MIMOSINE | C8 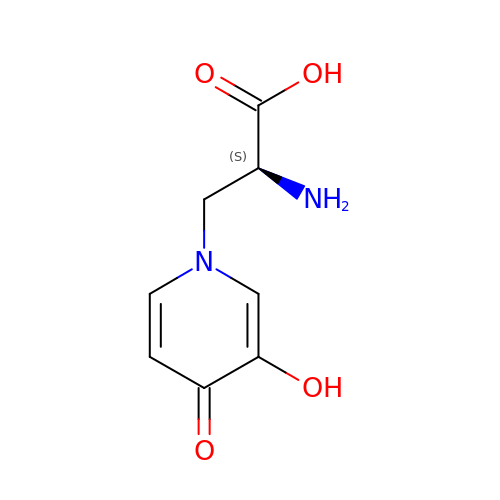H10 N2 O4 | WZNJWVWKTVETCG-YFKPBYRVSA-N>MAGYTELEKLHIMRDYLLPKQMEEHGLGRDKLQMNEEAMLKVIRQYTREAGVRNLNREA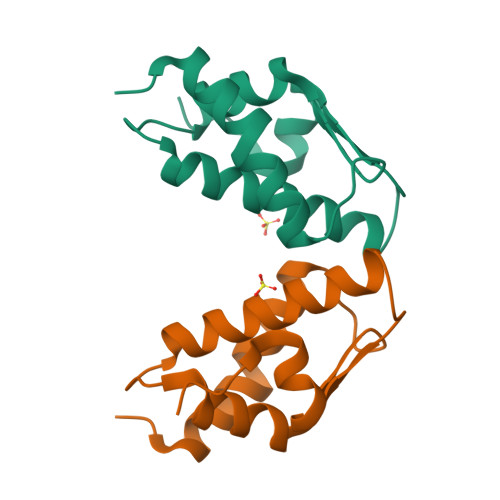ANICRKAARLIVSGEKKRVVVTPKTVESLLGKPRYRYGLAEREDQVGAVTGLAWTQALEHHHHHH[2x]> SPSAEACGYSDRVAQLTIGNSTITTQEAANIIVGYGEWPSYCSDSDATAVDKPTRPDVSVNRFYTLDTKLWEKSSKGWYWKFPDVLTETGVFGQNAQFH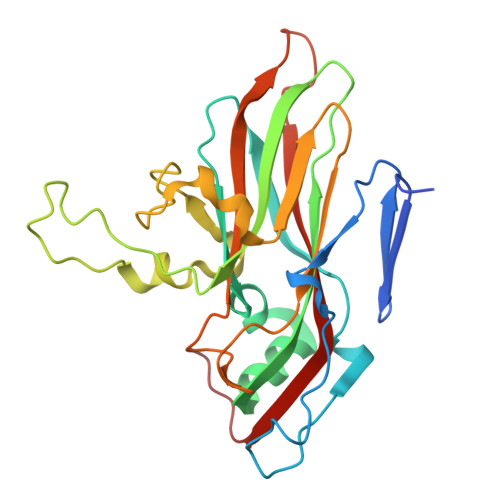YLYRSGFCIHVQCNASKFHQGALLVAVLPEYVIGSVAGGTGTEDTHPPYKQTQPGADGFELQHPYVLDAGIPISQLTVCPHQWINLRTNNCATIIVPYINALPFDSALNHCNFGLLVVPISPLDYDQGATPVIPITITLAPMCSEFAGLRQAVTQ> MDSAITLWQFLLQLLQKPQNKHMICWTSNDGQFKLLQAEEVARLWGIRKNKPNMNYDKLSRALRYYYVKNIIKKVN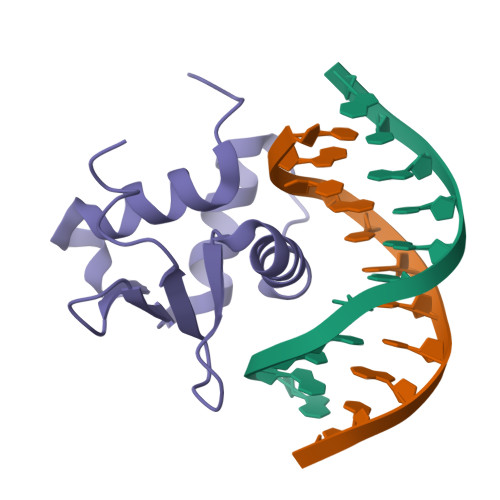GQKFVYKFVSYPEILNM>[16x]MRSSHHHHHHSSGLVPRGSHMESKKDDTDLKLVSHNVYMLSTVLYPNWGQYKRADLIGQSSYIKNNDVVIFNEAFDNGASDKLLSNVKKEYPYQTPVLGRSQSGWDKTEGSYSSTVAEDGGVAIVSKYPIKEKIQHVFKSGCGFDNDSNKGFVYTKIEKNGKNVHVIGTHTQSEDSRCGAGHDRKIRAEQMKEISDF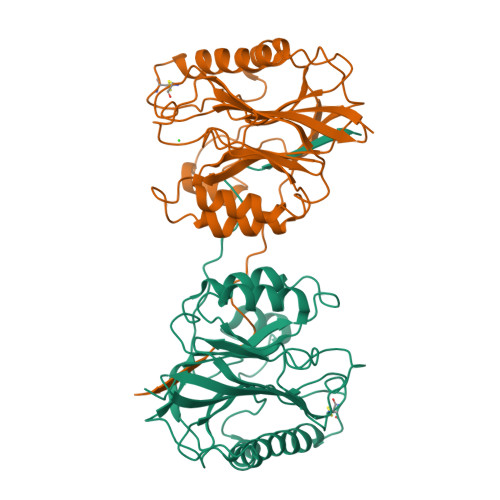VKKKNIPKDETVYIGGDLNVNKGTPEFKDMLKNLNVNDVLYAGHNSTWDPQSNSIAKYNYPNGKPEHLDYIFTDKDHKQPKQLVNEVVTEKPKPWNDFSDHYPIKAYSK> AKLDKEQVIDNALILLNEVGMEGLTTRKLAQKLGVEQPTLYWHVKNKRALLDALAETILQKHHHHVLPLANESWQDFLRNNAKSFRQALLMYRDGGKIHAGTRPSAN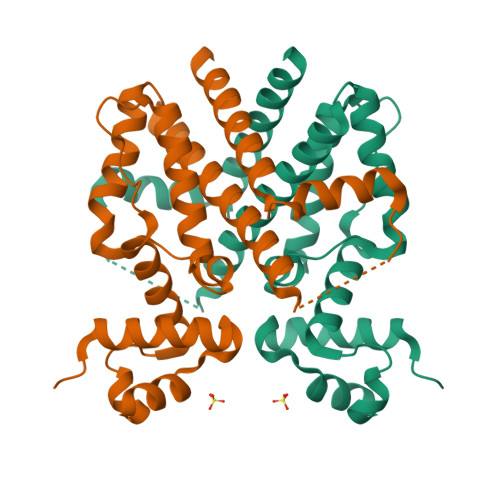QFETSEQQLQFLCDAGFTLTQAVYALSSIAHFTLGSVLETQEHQESQKEREKVPKTEINYPPLLTQAIDIMDSDNGEAAFLFVLDVMISGLETVLNNHH>[4x]SLKGKIEWVRVSAVVHSTEDREKVGEAISTLFPFEFEIAVSKAKGHYGNPMEYLEVELTKSSEIKKFWKNLLELLGEQAEEILSTLEDRIDEQNVLHIR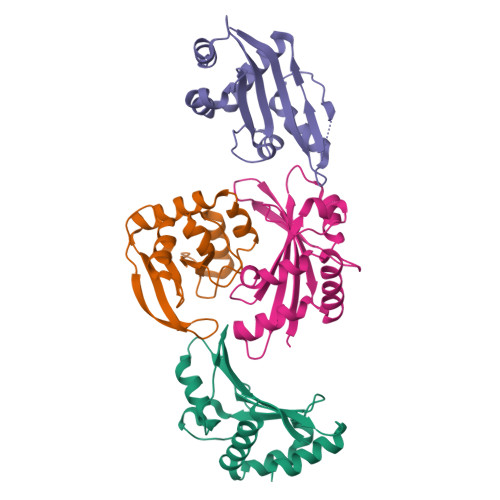IDKQKAYLGEVSLTSGGDPIAVKLRLVTYPSKREKVIEFARELCTIS>[4x]NPTSLTDVRVDKAVNFIKPEVSGVAEIQTVTGLSPSTSYLLTPAFLEQNFQSEAGIYILSATPVEGEGTISINMDPTVTTVSGFIKVKTDTFGTFDLSVVLTTASKKQTTGFNIIAATS

A major factor that limits the expansion of shrimp cultures is, however, infectious diseases from viruses, such as P. vannamei nodavirus (PvNV) and M. rosenbergii nodavirus (MrNV), which have inflicted heavy economic losses. The Nodaviridae genome comprises two single-stranded positive-sense RNA that encode the capsid protein for viral capsid assembly, the RNA polymerase for RNA replication, and the B2 protein for host RNA interference suppressor. While the shell domains (S-domains) of PvNV and MrNV contain conserved sequences of 62% identity, the protrusion domains (P-domains) and N-arms show low sequence identities of only 17% and 43%, respectively. In this work, we have determined the cryo-EM structures of T = 3 and T = 1 PvNV-LPs at atomic resolution, the crystal structures of the P-domains of PvNV and MrNV (PvNVPd and MrNVPd), and the crystal structure of the S-domain of PvNV (ΔN-ARM-PvNVSd) in the T = 1 subviral particle (SVP).

The PvNVPd forms dimers in two crystal forms with the asymmetric unit containing one dimer (space group P21) and two dimers (P212121). All structures of the PvNVPd were refined to resolutions 1.17–1.22 Å. The structures of PvNVPd from two crystal forms are similar with a root mean square deviation (RMSD) < 0.3 Å; and residues 250–368 were resolved in both structures. First, the crystal packing of PvNVPd (P212121) reflects the intermolecular organization of the two P-domain dimers with a bending angle of ~110°, suggesting that the existence of this putative conformation in the T = 3 PvNV virions arises from the simultaneous rotation of A/B dimer and the translation of C/C dimer. In the interface of this parallel model, the three turns β1/β2, β6/β7, and β7/β8 from one PvNVPd monomer are in close proximity to those of one symmetry molecule in the absence of metal ions. Notably, the sequence of the interaction region (Gln273–Asp278) of MrNVPd is distinct from that of PvNVPd, and two types (P21 and P212121) of PVNVPd structures do not exhibit the X-shaped conformation.>GLECDGRTNLCCRQQFFIDFRLIGWNDWIIAPTGYYGNYCEGSCPAYLAGVPGSASSFHTAVVNQYRMRGLNPGTVNSCCIPTKLSTMSMLYFDDEYNIVKRDVPNMIVEECGCA[3x];>[3x]SQ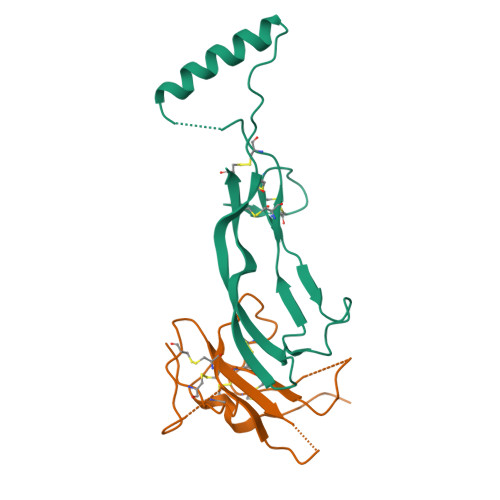NQERLCAFKDPYQQDLGIGESRISHENGTILCSKGSTCYGLWEKSKGDINLVKQGCWSHIGDPQECHYEECVVTTTPPSIQNGTYRFCCCSTDLCNVNFTENFPPPDTT>SQQQ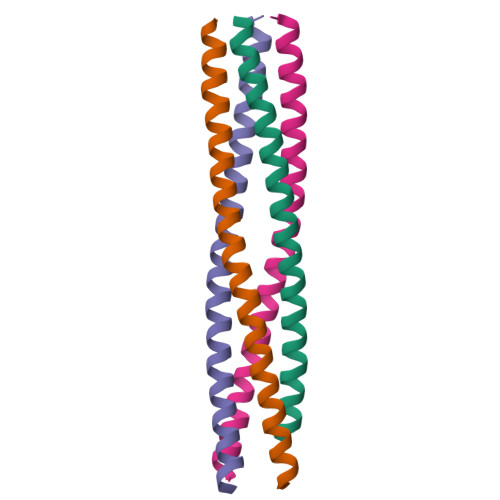IAALSESLQATQQQLQALQQQCYELEKTNRLLVSEVMTLQKMVKAQNQASNEIINHL[4x]>[2x]TTRSWDFLGFPLTVPRRSQVESNIVVGVLDTGIWPESPSFDDEGFSPPPPKWKGTCETSNNFRCNRKIIGARSYHIGRPISPGDVNGPRDTNGHGTHTASTAAGGLVSQANLYGLGLGTARGGVPLARIAAYKVCWNDGCSDTDILAAYDDAIADGVDIISLSVGGANPRHYFVDAIAIGSFHAVERGILTSNSAGNGGPNFFTTASLSPWLLSVAASTMDRKFVTQVQIGNGQSFQGVSINTFDNQYYPLVSGRDIPNTGFDKSTSRFCTDKSVNPNLLKGKIVVCEASFG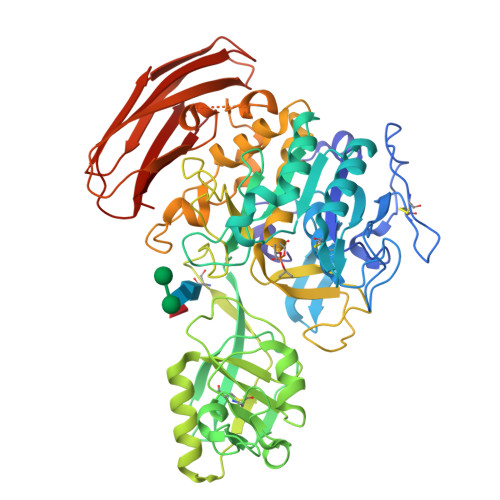PHEFFKSLDGAAGVLMTSNTRDYADSYPLPSSVLDPNDLLATLRYIYSIRSPGATIFKSTTILNASAPVVVSFSSRGPNRATKDVIKPDISGPGVEILAAWPSVAPVGGIRRNTLFNIISGTSMSCPHITGIATYVKTYNPTWSPAAIKSALMTTASPMNARFNPQAEFAYGSGHVNPLKAVRPGLVYDANESDYVKFLCGQGYNTQAVRRITGDYSACTSGNTGRVWDLNYPSFGLSVSPSQTFNQYFNRTLTSVAPQASTYRAMISAPQGLTISVNPNVLSFNGLGDRKSFTLTVRGSIKGFVVSASLVWSDGVHYVRSPITITSLV> IESIIKTATDTVKSEINAELGVVPSLNAVETGASSNTEPEEAIQTRTVINQHGVSETLVENFLSRAALVSKRSFEYKNHTSSEARTDKNFYKWTINTKSFVQLRRKLELFTYLRFDAEITILTTVAVGSNNSTYMGLPDLTLQAMFVPTGALTPEKQDSFHWQSGSNASVFFKVSDPPARMTIPFMCINSAYSVFYDGFAGFEKNGLYGINPADTIGNLCVRIVNEHQPIGFTVTVRVYMKPKHIKAWAPRPPRTLPYMSIANANYKGKERAPNALNAIIGNRESVKTMPHDIRLV;> MGAQVTR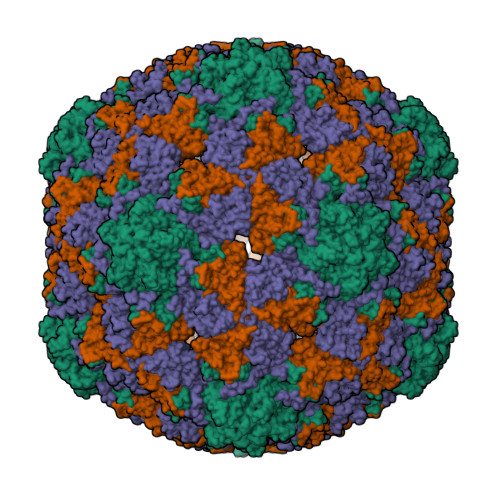QQTGTHENANIATNGSHITYNQINFYKDSYAASASKQDFSQDPSKFTEPVVEGLKAGAPVLKSPSAEACGYSDRVLQLKLGNSAIVTQEAANYCCAYGEWPNYLPDHEAVAIDKPTQPETATDRFYTLKSVKWETESTGWWWKLPDALNNIGMFGQNVQHHYLYRSGFLIHVQCNATKFHQGALLVVAIPEHQRGAHNTTTSPGFDDIMKGEEGGTFNHPYVLDDGTSLACATIFPHQWINLRTNNSATIVLPWMNAAPMDFPLRHNQWTLAIIPVVPLGTRTVSSMVPITVSIAPMCCEFNGLRHAITQ;> GVPTYLLPGSGQFLTTDDHSSAPVLPCFNPTPEMHIPGQVRNMLEVIQVESMMEINNTENAVGMQRLKVDISVLTDVDQLLFNIPLDIQLDGPLRNTLVGNISRYYTHWSGSLEMTFMFCGSFMATGKLILCYTPPGGSCPTTRETAMLGTHIVWDFGLQSSVTLVIPWISGSHYRMFNNDAKSTNANVGYVTCFMQTNLIVPSESSNTCSLIGFVAAKDDFSLRLMRDSPDIGQLEHLHEAEAAYQ>AKRKRIEMYTKASFKASNQKIEQIWKTQQEEIQKLNNEYSQQFMNVLQQWELDIQKFEEQGEKLSNLFRQQQKIFQQSRIVQSQRMKAIKQIHEQFIKSLEDVEKNNDNLFTGTQSELKKEMAMLQKKVMMETQQQEMANVRKS[4x]

A highly-conserved meiosis-specific structure, the chromosome axis, assembles in early meiotic prophase and provides a scaffold for the organization of chromosomes as a linear array of loops, and also orchestrates the formation of DSBs and their repair as inter-homolog crossovers. Mammals possess two such proteins, SYCP2 (1500 residues in Mus musculus) and SYCP3 (254 residues), which are both required for proper axis formation and wild-type levels of crossovers, and are known to interact with one another through their C-terminal coiled-coil domains. Mammalian SYCP3 is known to form coiled-coil homotetramers that self-associate into larger structures both in cell culture and in vitro, but how SYCP3 cooperates with SYCP2 to mediate chromosome localization and axis assembly is not known. We further show that both SYCP2/SYCP3 and ASY3/ASY4 form heterotetrameric coiled-coil complexes that self-assemble into extended filaments, paralleling our findings with Red1.

We combined the truncations on both proteins to yield a minimal construct, Mm SYCP21325-1479:SYCP3105-248, which we term SYCP2CC:SYCP3CC hereon. We found that Mm SYCP3CC also forms homotetramers in the absence of SYCP2CC (not shown), and when we determined the structure of Mm SYCP3CC by x-ray crystallography, we observed an antiparallel coiled-coil homotetramer similar in structure to H. sapiens SYCP3. As SYCP2 and SYCP3 share limited sequence homology in their coiled-coil region, we reasoned that SYCP3 homotetramers may form through promiscuous coiled-coil interactions in the absence of SYCP2. To compare the stability of Mm SYCP3CC homotetramers with Mm SYCP2CC:SYCP3CC heterotetramers, we measured their melting temperatures (Tm) using a dye-binding assay. We found that the SYCP2CC:SYCP3CC heterotetramer is more stable than SYCP3CC on its own (56.0°C Tm versus 52.5°C), supporting the idea that the heterotetrameric complex is the preferred state when both proteins are present. While the SYCP3CC homotetramer is likely not the favored state in the presence of SYCP2, its structure may nonetheless be informative as to the structure of SYCP2CC:SYCP3CC. Overall, these data show that the SYCP2CC:SYCP3CC complex forms an extended coiled-coil tetramer with an overall structure similar to that of the SYCP3 homotetramer. Using sequence alignments and the structures of H. sapiens and M. musculus SYCP3, we generated physical models for SYCP2:SYCP3 where the monomers are arranged either parallel or antiparallel, and mapped all identified crosslinks onto these models. In agreement with our SAXS data, the crosslinking data strongly support a heterotetramer model with two SYCP2 monomers arranged parallel to one another and antiparallel to two SYCP3 monomers.> ADGIQSRKTYTLTDYLKNTYRLKLYSLRWISDHEYLYKQENNILVFNAEYGNSSVFLENSTFDEFGHSINDYSISPDGQFILLEYNYVKQWRHSYTASYDIYDLNKRQLITEERIPNNTQWVTWSPVGHKLAYVWNNDIYVKIEPNLPSYRITWTGKEDIIYNGITDWVYEEEVFSAYSALWWSPNGTFLAYAQFNDTEVPLIEYSFYSDESLQYPKTVRVPYPKAGAVNPTVKFFVVNTDSLSSVTNATSIQITAPASMLIGDHYLCDVTWATQERISLQWLRRIQNYSVMDICDYDESSGRWNCLVARQHIEMSTTGWVGRFRPSEPHFTLDGNSFYKIISNEEGYRHICYFQIDKKDCTFITKGTWEVIGIEALTSDYLYYISNEYKGMPGGRNLYKIQLSDYTKVTCLSCELNPERCQYYSVSFSKEAKYYQLRCSGPGLPLYTLHSSVNDKGLRVLEDNSALD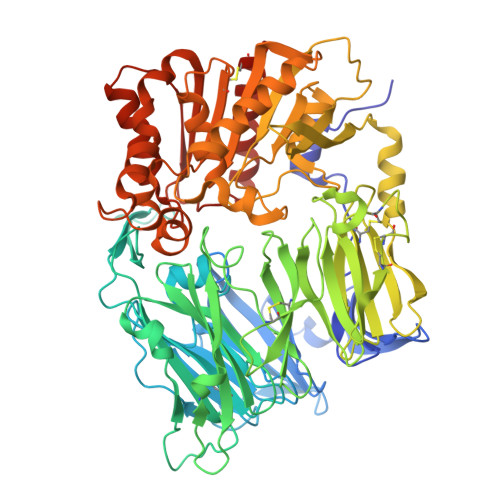KMLQNVQMPSKKLDFIILNETKFWYQMILPPHFDKSKKYPLLLDVYAGPCSQKADTVFRLNWATYLASTENIIVASFDGRGSGYQGDKIMHAINRRLGTFEVEDQIEAARQFSKMGFVDNKRIAIWGWSYGGYVTSMVLGSGSGVFKCGIAVAPVSRWEYYDSVYTERYMGLPTPEDNLDHYRNSTVMSRAENFKQVEYLLIHGTADDNVHFQQSAQISKALVDVGVDFQAMWYTDEDHGIASSTAHQHIYTHMSHFIKQCFSLPHHHHHH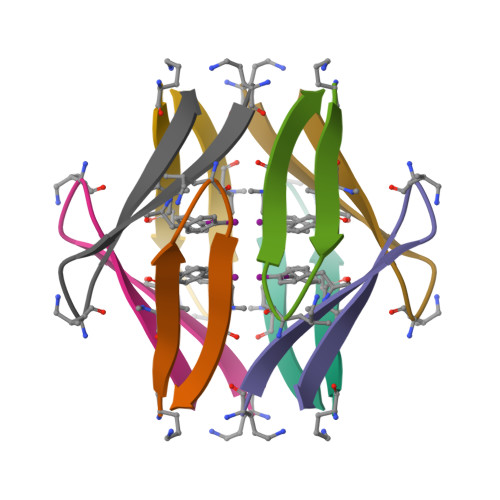> AYLLFYTELKVTVTVK>[4x]GAMDPQFMKKVAVIDIEGTLTDFEFWREMARITGKREIEELLEKGLSGEVEWLDSLLKRVGLIRGIDEGTFLRTREKVNVSPEARELVETLREKGFKVV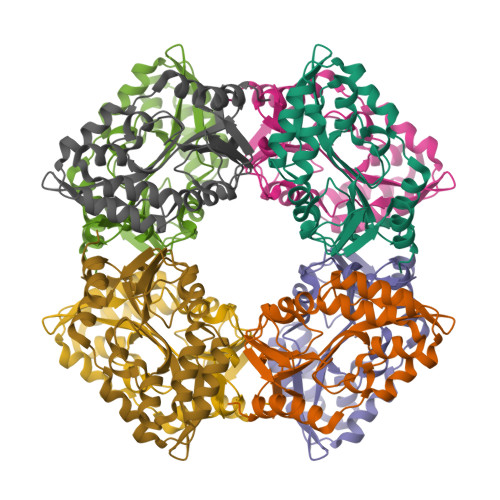LISGSFEEVLEPFKELGDEFMANRAIFEDGKFQGIRLRFRDKGEFLKRFRDGFILAMGDGYADAKMFERADMGIAVGREIPGADLLVKDLKELVDFIKNLKP> MSQDSPDGQYENSEGGWMEDYDYVHLQGKEEFEKTQKELLEKG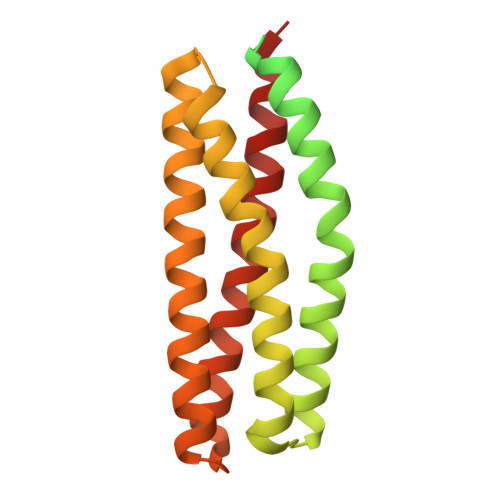SITRQGKSQLELQQLKQFERLEQEVSRPIDHDLANWTPAQPLAPGRTGGLGPSDRQLLLFYLEQCEANLTTLTNAVDAFFTAVATNQPPKIFVAHSKFVILSAHKLVFIGDTLSRQAKAADVRSQVTHYSNLLCDLLRGIVATTKAAALQYPSPSAAQDMVERVKELGHSTQQFRRVLGQLAAALE> PKLLNKFDKTIKAELDAAEKLRKRGKIEEAVNAFKELVRKYPQSPRARYGKAQCEDDLAEKRRSNEVLRGAIETYQEVASLPDVPADLLKLSLKRRSDRQQFLGHMRGSLLTLQRLVQLFPNDTSLKNDLGVGYLLIGDNDNAKKVYEEVLSVTPNDGFAKVHYGFILKAQNKIAESIPYLKEGIESGDPGTDDGRFY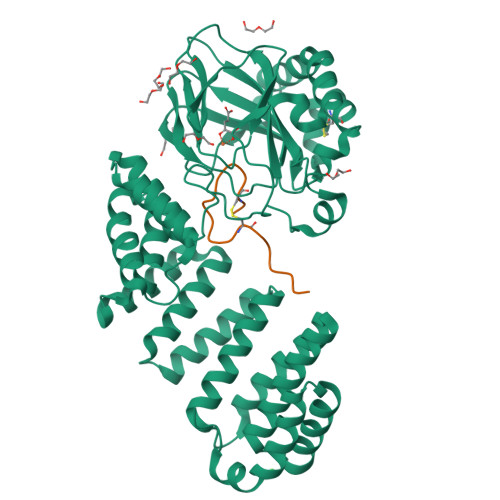FHLGDAMQRVGNKEAYKWYELGHKRGHFASVWQRSLYNVNGLKAQPWWTPKETGYTELVKSLERNWKLIRDEGLAVMDKAKGLFLPEDENLREKGDWSQFTLWQQGRRNENACKGAPKTCTLLEKFPETTGCRRGQIKYSIMHPGTHVWPHTGPTNCRLRMHLGLVIPKEGCKIRCANETKTWEEGKVLIFDDSFEHEVWQDASSFRLIFIVDVWHPELTPQQRRSLPAI;> DGDQSETSPSQNQGKCKNGLGEYTCTSLEGFEGKNSELF~{N}-[(1~{R},2~{R})-7-chloranyl-2-oxidanyl-1,2,3,4-tetrahydronaphthalen-1-yl]-4-ethanoyl-3-ethyl-5-methyl-1~{H}-pyrrole-2-carboxamide | C20 H23 Cl N2 O3 | 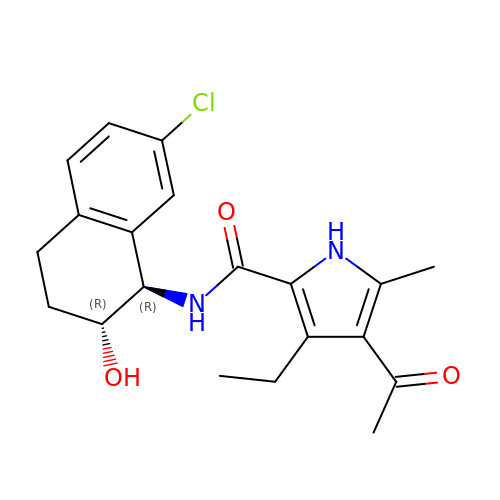KVJAGYRUNZONPJ-SJLPKXTDSA-N> MKHHHHHHPMSGLVPRGSAMGEPLASASKFSSIVSNDIDMNFRSFKFWVHNDNLMEVKTR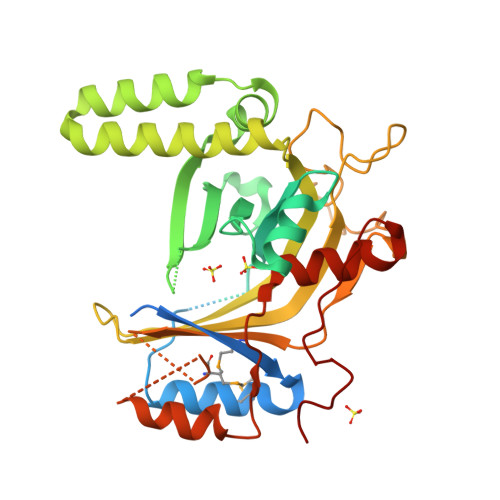ILRHLPVLVYANVPSENDDLVNRFESDISNNDEIVGSSSSTSSVEHGLGARSFDPLINTLYFDNEHFELYNDKLLKLNSAPTLRLRWTGQLSDKPDIFLEKKTLIEDEATGKSEFDLTKLQLKQKFINGFIFEGDKKFKEQTLKKLKESGTAGRDLERLEEDFSEIQNFIIKNELQPVFRTVYTRTAFQIPGDDKIRVTIDSNIVFIKEDSFDRERPIRDPNTWHRTDIDANVANPLKFLRGGEYAKFPYSVMEIKVKSSLDSSMSASSMISNVKLPKKHGQWLNDLTNSHLVKEIPKFSIFVQGVASLYGDDEKLDILPFWLPDLETDIRQ>MAPVEFPKSLRASSHSSEGGTTKEEDIYGYELLYRSAFASYIAPTGAWNLVWFQAADGSIKQARWYGEWVISTVLAPGKALQGTPLTALLWGPQDTVRLYYLSPQFELQEWCWDTKNGADNKYDGALNAAKVKVAPYSKLGAVSFGGANLRVYYQG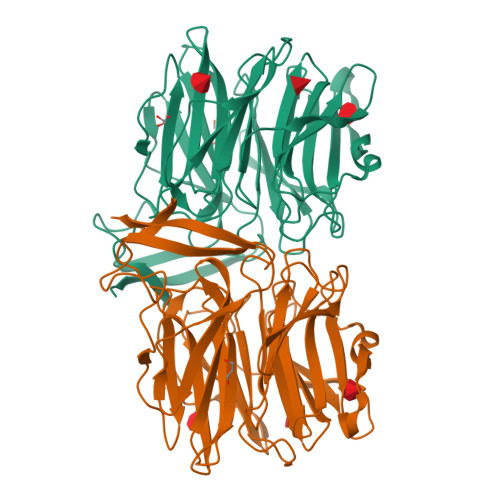TNNKLEEYTFGGGQGWKKGATLPGDPLPGTYISFVNRNKWDANPPSIRGYFQTVTGSLAEQVWETGGWRIGQFVIPAAPFLTPISATVSPEKDFPKIHVYWLSVESTIIESVNWHGWKAPKQIDNISVVKADISATSFTRDDGTVDVRIYGTAQLNVLFERIFRYGVWEEKIHSISVGKEIPIEVVGVAAALEHHHHHH[2x]> MNYNPEEQFRCTIIRGKAKNMLDNLLPAYANIIDDICPCDKASFVKDFNNRLIEILGEETTKKTLDNHRTEIAGKLFGMFYEDDEVIFPSGRTNKYIEDSDQPAFFKDICFKFQFPNGMDKLDKVIEKVGAKIQIRQFPYILQVLLTADNNNIQLSKDDIAYYVLNSLQVLQGKIKPIEVIEKIIEDRSNDITKKVRHPGKETSYSMQHIREQLNYLELANLIRIDGNLVKLNYREAENINYIAQFWGNKPEFNAYKYDFTSEDDKK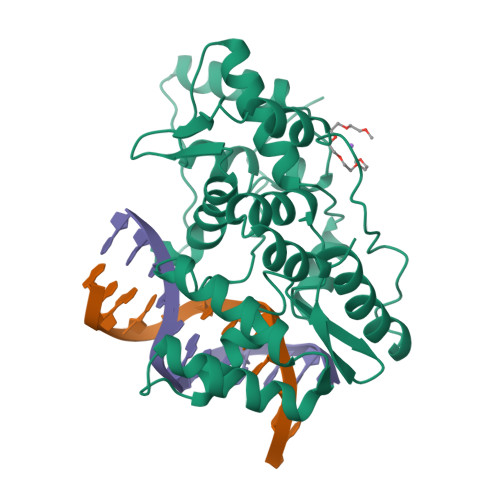SFFKDWQQYYSNVNSHKS>[2x]GQLSYKSMHLTPFTLSALLASFHKVEVLNLNGLQIEEIDTNAFAYAHTIQKLYMRFNVIRYLPPHVFQNVPLLTVLMLDRNDLSSLPPGIFHNTPKLTMMSMSNNNLERIEDDTFQATTALQNLQLSSNRLTHVDLALIPSLFHVNVSYNLLSTLAIPIAVEELDASHNTINVVRGPVNVELTILKLQHNNLTDTAWLLNYP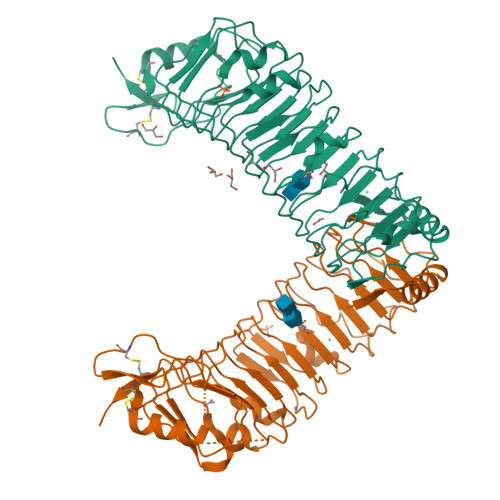GLVDVDLSYNQLEKITYQHFVKMQRLERLYVSNNRLVALDFYGRPIPTLKVLDLSHNHLMWVEHNQAQFDKLQYLYLDHNSIVTFKLSTSHTLKNLTLSHNDWDCNSLRALFRNVAQPAVHDADQHCKIDYHLEHGLCCKESDKPYLDHHHHHH> GRHG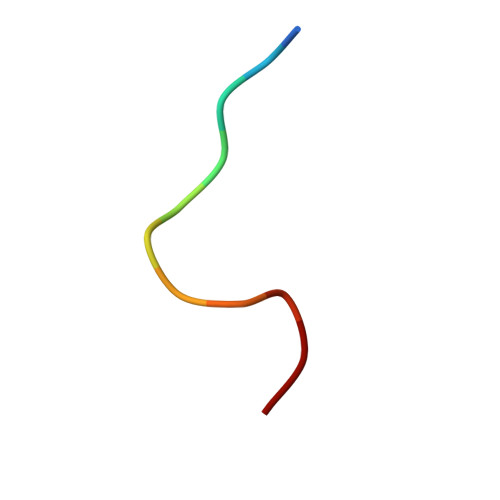AANDENY>GAMAPHFKEELRNLNVRYQSNATLVCKVTGHPKPIVKWYRQGKEIIADGLKYRIQEFKGGYHQLIIASVTDDDATVYQVRATNQGGSVSGTASLEVEVPAKIHLPKTLEGMGAVHALRGEVVSIKIPFSGKPDPVITWQKGQDLIDNNGHYQVIVTRSFTSLVF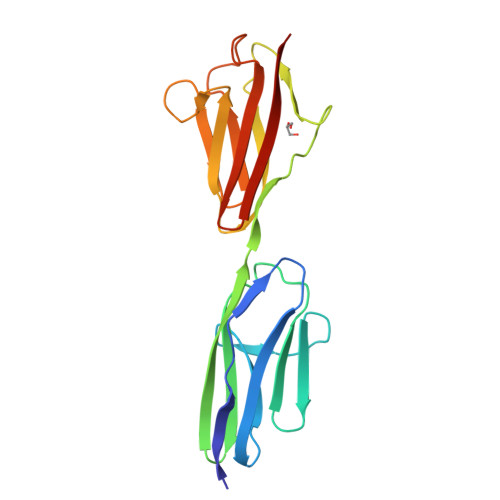PNGVERKDAGFYVVCAKNRFGIDQKTVELDVAD[2x]>[2x]GAMDPGNSAEAWYNLGNAYYKQGDYDEAIEYYQKALELDPNNAEAWYNLGNAYYKQGDYDEAIEYY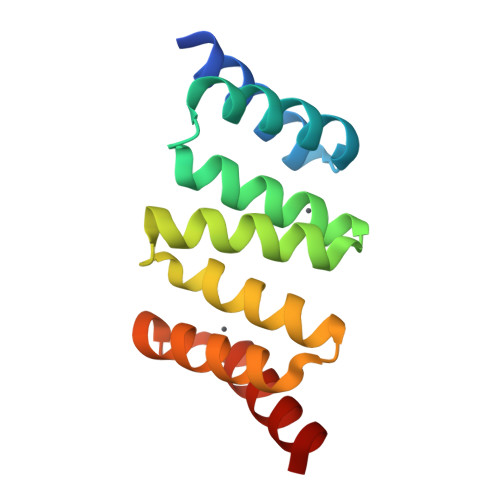QKALELDPNNAEAWYNLGNAYYKQGDYDEAIEYYQKALELDPNNAEAKQNLGNAKQKQG>[8x]MRGSHHHHHHLVPRGSKTRGQIQVILGPMFSGKSTELMRRVRRFQIAQYKCLVIKYAKDTRYSSSFCTHDRNTMEALPACLLRDVAQEALGVAV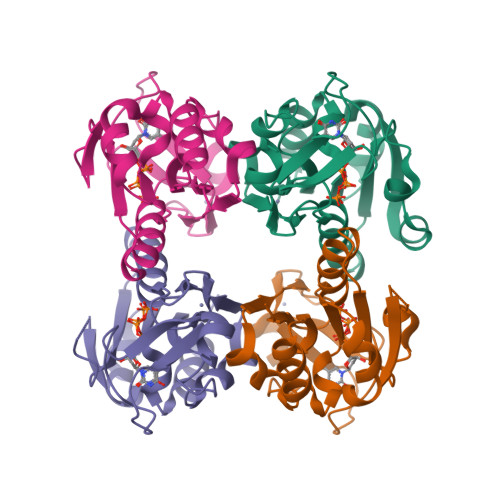IGIDEGQFFPDIVEFCEAMANAGKTVIVAALDGTFQRKPFGAILNLVPLAESVVKLTAVCMECFREAAYTKRLGTEKEVEVIGGADKYHSVCRLCYFKKAS>[2x]HHHHHHSSGHIDDDDKMAPSILSTESSIIVIGAGTWGCSTALHLARRGYKDVTVLDPHPVPSPIAAGNDINKIMEHSELKDGSSDPRSAAFSTFTRAALKAWKTDPVFQPYFHETGFIISGHTPALIDHIRKDEVEPSETNFVKLETAEDFRRTMPPGVLTGDFPGWKGWLHKSGAGWIHAKKAMISAFNEAKRLGVRFVTGSPEGNVVSLVYEDGDVVGARTADGRVHKA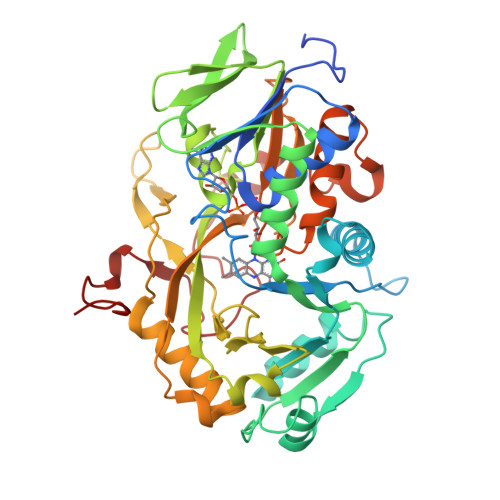HRTILSAGAGSDSLLDFKKQLRPTAWTLCHIQMGPEEVKQYRNLPVLFNIAKGFFMEPDEDKHELKICDEHPGYCNFLPDPNRPGQEKSVPFAKHQIPLEAEARARDFLHDTMPHLADRPLSFARICWDADTPDRAFLIDRHPEHPSLLVAVGGSGNGAMQMPTIGGFIADALESKLQKEVKDIVRWRPETAVDRDWRATQNRFGGPDRIMDFQQVGEDQWTKIGESRGP1-(biphenyl-3-yl)-1H-imidazole 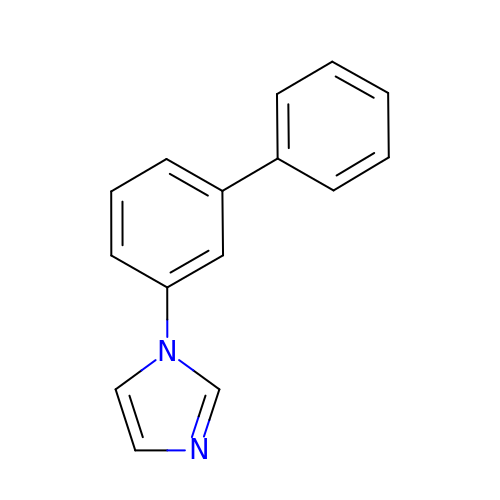| C15 H12 N2 | HGZNKHJCDHAXJE-UHFFFAOYSA-N>[3x]SDPA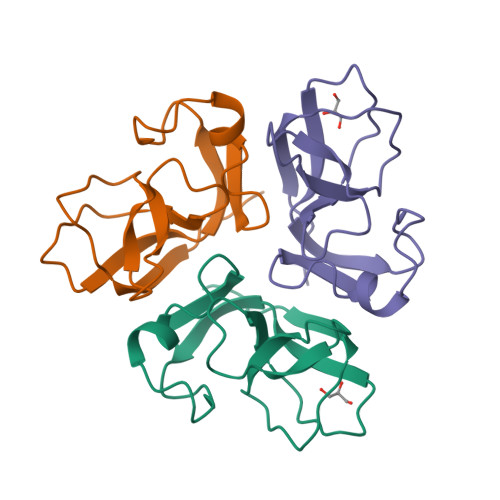HTATAPGGLSAKAPAMTPLMLDTSSRKLVAWDGTTDGAAVGILAVAADQTSTTLTFYKSGTFRYEDVLWPEAASDETKKRTAFAGTAISIV>[4x]MSQHNEKNPHQHQSPLHDSSEAKPGMDSLAPEDGSHRPAAEPTPPGAQPTAPGSLKAPDTRNEKLNSLEDVRKGSENYALTTNQGVRIADDQNSLRAGSRGPTLLEDFILREKITHFDHERIPERIVHARGSAAHGYFQPYKSLSDITKADFLSDPNKITPVFVRFSTVQGGAGSADTVRDIRGFATKFYTEEGIFDLVGNNTPIFFIQDAHKFPDFVHAVKPEPHWAIPQGQSAHDTFWDYVSLQPETLHNVMWAMSDRGIPRSYRTMEGFGCHTFRLINAEGKATFVRFHWKPLAGKASLVWDEAQKLTGRDPDFHRRELWEAIEAGDFPEYELGFQLIPEEDEFKFDFDLLDPTKLIPEELVPVQRVGKMVLNRNPDNFFAENEQAAFHPGHIVPGLDFTNDPLLQGRLFSYTDTQISRLGGPNFHEIPINRPTAPYHNFQRDGMHRMGIDTNPANYEPNSINDNWPRETPPGPKRGGFES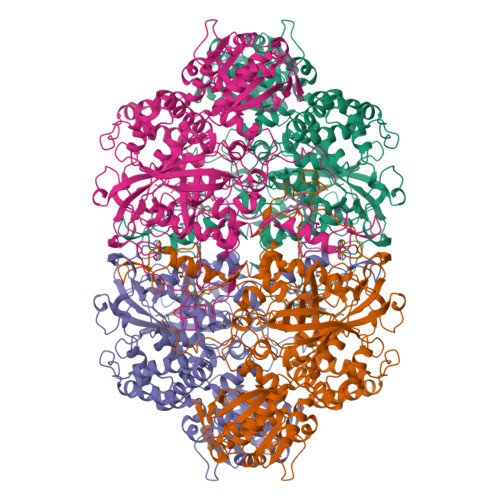YQERVEGNKVRERSPSFGEYYSHPRLFWLSQTPFEQRHIVDGFSFELSKVVRPYIRERVVDQLAHIDLTLAQAVAKNLGIELTDDQLNITPPPDVNGLKKDPSLSLYAIPDGDVKGRVVAILLNDEVRSADLLAILKALKAKGVHAKLLYSRMGEVTADDGTVLPIAATFAGAPSLTVDAVIVPAGNIADIADNGDANYYLMEAYKHLKPIALAGDARKFKATIKIADQGEEGIVEADSADGSFMDELLTLMAAHRVWSRIPKIDKIPA> MEYEWKPDEQGLQQILQLLKE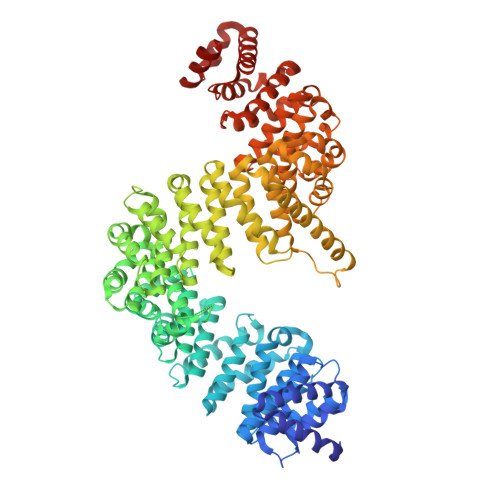SQSPDTTIQRTVQQKLEQLNQYPDFNNYLIFVLTKLKSEDEPTRSLSGLILKNNVKAHFQNFPNGVTDFIKSECLNNIGDSSPLIRATVGILITTIASKGELQNWPDLLPKLCSLLDSEDYNTCEGAFGALQKICEDSAEILDSDVLDRPLNIMIPKFLQFFKHSSPKIRSHAVACVNQFIISRTQALMLHIDSFIENLFALAGDEEPEVRKNVCRALVMLLEVRMDRLLPHMHNIVEYMLQRTQDQDENVALEACEFWLTLAEQPICKDVLVRHLPKLIPVLVNGMKYSDIDIILLKGDVEGGSGGSGDDTISDWNLRKCSAAALDVLANVYRDELLPHILPLLKELLFHHEWVVKESGILVLGAIAEGCMQGMIPYLPELIPHLIQCLSDKKALVRSITCWTLSRYAHWVVSQPPDTYLKPLMTELLKRILDSNKRVQEAACSAFATLEEEACTELVPYLAYILDTLVFAFSKYQHKNLLILYDAIGTLADSVGHHLNKPEYIQMLMPPLIQKWNMLKDEDKDLFPLLECLSSVATALQSGFLPYCEPVYQRCVNLVQKTLAQAMLNNAQPDQYEAPDKDFMIVALDLLSGLAEGLGGNIEQLVARSNILTLMYQCMQDKMPEVRQSSFALLGDLTKACFQHVKPCIADFMPILGTNLNPEFISVCNNATWAIGEISIQMGIEMQPYIPMVLHQLVEIINRPNTPKTLLENTAITIGRLGYVCPQEVAPMLQQFIRPWCTSLRNIRDNEEKDSAFRGICTMISVNPSGVIQDFIFFCDAVASWINPKDDLRDMFCKILHGFKNQVGDENWRRFSDQFPLPLKERLAAFYGV ADP-ribosylation is a reversible post-translational modification involved in various cellular activities. Removal of ADP-ribosylation requires (ADP-ribosyl)hydrolases, with macrodomain enzymes being a major family in this category. Further analyses reveal DUF4804 as a class of MavL-like macrodomain enzymes whose representative members show unique selectivity for mono-ADP-ribosylated arginine residue in synthetic substrates. Crystal structures of several proteins in this class provide insights into arginine specificity and a shared mode of ADP-ribose interaction distinct from previously characterized macrodomains.

Two of the representative proteins in this group, CG2909, and CG3568, are from Drosophila melanogaster, indicating potential evolutionary connections between the prokaryotic effector and the eukaryotic proteins. Encouraged by the clearly detectable ADPR-Ub hydrolytic activity of the two metazoan proteins, we solved their crystal structures in the ADPR-bound forms (ADPR-bound CG290912-498 at 2.28 Å and the ADPR-bound CG356825-508 at 2.00 Å). The ADPR interactions in both CG2909 and CG3568 are similar to those observed in MavL, with di-phosphate-binding loops and catalytic loops matching the sequence motifs identified from our search. In addition, water molecules equivalent to w4 in MavL can be found in both structures with distances of 3.4 Å (in CG2909) and 3.3 Å (in CG3568), suggesting that this macrodomain class likely employs a similar catalytic mechanism. Adenosines in MavL, CG2909, and CG3568 are sandwiched between two residues and stabilized by π-π (in MavL) or π-π and π-cation (in CG2909 and CG3568) interactions. In MavL, the adenosine was stabilized by π-π stacking interaction provided by two aromatic residues (H142 and Y265), whereas in the two Drosophila proteins, a π-cation interaction involving an arginine (R198 in CG2909 and R209 in CG3568) replaces the imidazolium stacking. In Arg-specific macrodomains, the core β-strand connectivity appears to be the same, yet some distinct differences are observed: In both CG2909 and CG3568, expansion of the variable regions from β7 to β9 (compared to β4–β5 in MavL) and the additional β12–β13 were observed. Interestingly, CG2909, CG3568, and Larg1 all harbor a hydrophobic residue (F137 in CG2909, F148 in CG3568, and V77 in Larg1) equivalent to F105 in MavL in their insertions. On the other hand, E107 in MavL also seems to have functionally equivalent residues in the other three enzymes (S226 in CG2909, E237 in CG3568, and E160 in Larg1), even though these residues are not in the insertions. On the other hand, our study also tapped into the protein-level specificity: MavL interacts with Ub and effectively removes ADPR from ADPR-Ub, whereas Larg1, CG2909, and CG3568 exhibited rather weak activity hydrolyzing ADPR-Ub.

>GPLGSWPAVTGDSPHLTNFGRKLLKDCRQVQKPIGGYENLGNVIKLSAEFPLEFGVNSVKVYRQSPSRLARINEEVASAYPLIHERTLGLYLQYLEHKCRWGNAVEKPIYRNLSLCGFVQRLLVKRCASFFARNDKYLLVSGESGASGFEAVGTREEKAPLVLANVLSYDDIKLSALLSVSSRTEFVNEGERTNCGHVDLNTKTLERHGVIVGMIGARLSRRNLMEFQDIVIARQQNTRERGYGMALDEPATTRDEDYRRLWREFYATRDLIHGQAVIDNQRFGPSKNKMDVFDNLVMKRRYAISFDMLLLEAEARAKRVKKLAYIHVVGFGLGVWKAAEQQERIFMETFEQRMRTLGNRLNNVGLVHFSWFSITHCGGLSNGSLIEIPGHPKDGIRVLISKRNPARKLSDPEHAGMLLVVSYAWDGNALPGNEFWMKMLQSTGDSSTACSTLVAELHNPYINTKFCNGGNLHIASPEHGVLHIAEYAKRVI[4x]> MATLEAMQVSEEQQSLIMEDVQVLLPNYDDFVEDVLQQFMEENPETFQIFPWADASKTAKEMR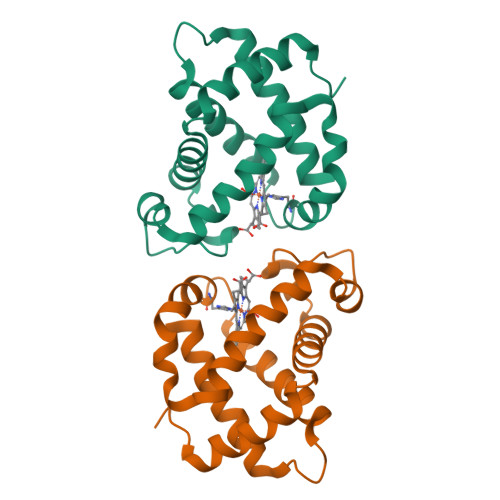SHPRFKSHAKSIGKVISDCLVDLNGVKKHEPKLSSLGAMHTKKKVPTELFGKLGGCILTQVVKRVSEAKWSEEKKEAWLKAYGIITVMVTE(3R,5S,9R,21S)-1-[(2R,3S,4R,5R)-5-(6-amino-9H-purin-9-yl)-4-hydroxy-3-(phosphonooxy)tetrahydrofuran-2-yl]-3,5,9,21-tetrahydroxy-8,8-dimethyl-10,14,19-trioxo-2,4,6-trioxa-18-thia-11,15-diaza-3,5-diphosphatricosan-23-oic 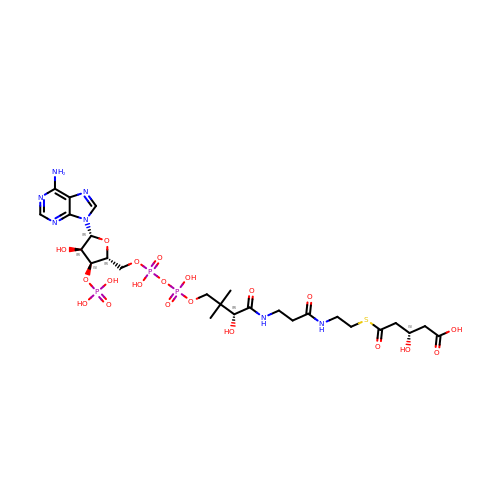acid 3,5-dioxide | C26 H42 N7 O20 P3 S | IIYZSYKTQRIPRG-UPWLPGGHSA-N PHOSPHORIC ACID 2,3-BIS-(3,7,11,15-TETRAMETHYL-HEXADECYLOXY)-PROPYL ESTER 2-HYDROXO-3-PHOSPHONOOXY-PROPYL ESTER | C46 H96 O11 P2 | 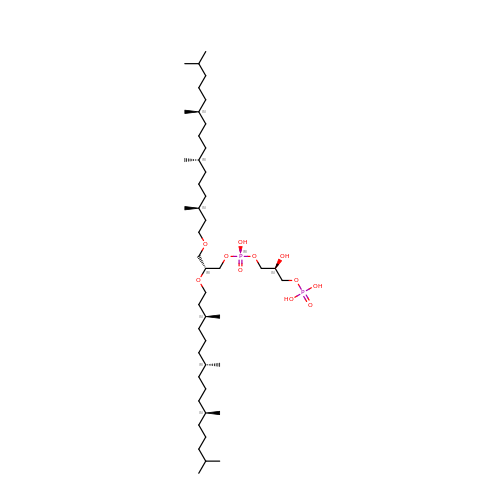TZXJQSKPTCRGCA-QVBLKRSVSA-N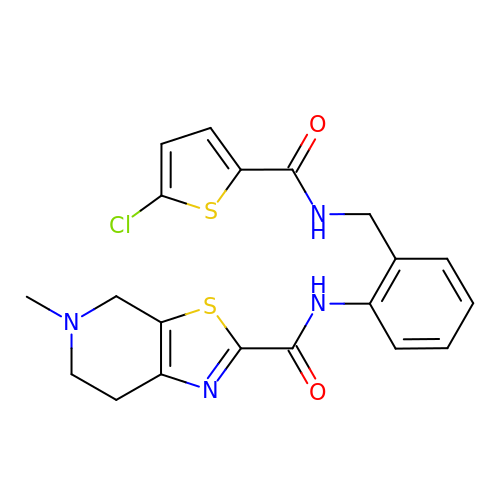N-[2-({[(5-chlorothiophen-2-yl)carbonyl]amino}methyl)phenyl]-5-methyl-4,5,6,7-tetrahydro[1,3]thiazolo[5,4-c]pyridine-2-carboxamide | C20 H19 Cl N4 O2 S2 | LMUFNFLXBDOGET-UHFFFAOYSA-N>[2x]SNAMLLYTKKDDIYSDIVRMILLIKGANAKIVDVSKEENSKHLEELNIITPNG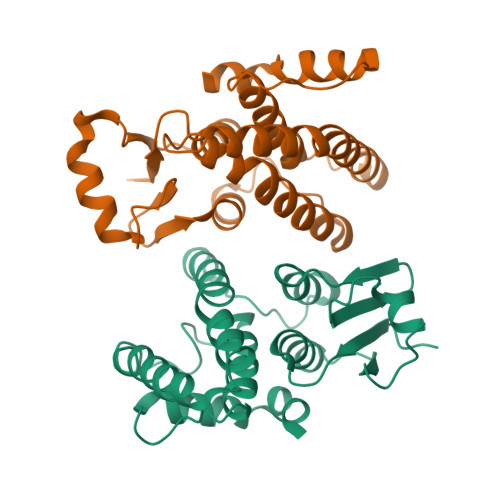NIPTLSTDDFAVYRLSVIIEAIEDLYPFPPMFPVFPKQRANARILLEYVNKTFLQNIIKLQSPDLDEKQANEIKMLMQRDIISTYKKIVSEREVNAESNPDAQNINVLTLIITFVFYYFIKLKISIPTKDKNIIKEIKELLSEPNFIKTIK;>SNAMVTLYTTKYCPYSLRARIALAEKKMSTDIVEAGDLEPAMIKKITPNGVFPVLMEKDYSINNRKALLIYIDERFPAPSLLPNVVNERIKIRLSLDKIDNEWYPVLDQIRKHRSDQKMLESMFKDLKESLLAMEKAFTGSEFFISSGFTLADCYIAALIICLEAEGFIIDDEYGAIYEYKKRLFARDSVKKANIKGGAGESLLKTLRTHR[2x]> HHHH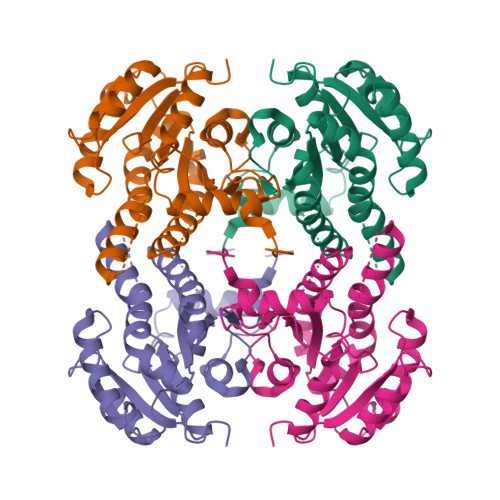HHENLYFQSMLLKGQRFVVTGIASKLSIAWAIAESLHREGAQLILTYPNDKIKKRVDMAAEAFDAVAVIECDVGSDESIQVCFDEIAKHWGVGDDKGIDGIVHAIGFAPADQLDGDFTQATTREGSQIAHDISSYSFVALAKAGRELLAARQGSLLTLTYEGSISVLPNYNVMGMAKASLEASVRYLASSLGGEGIRVNAISAGPIRTLAASGIKSFRRMLDVSEKIAPLQRNVSQEEVGNAALFLLSPWASGITGEILFVDAGFNTVAISEKIMMMAGDGEQ> VTKPYSSPPTNLRSLRDRLTQVAERQGVVFGRLQRHV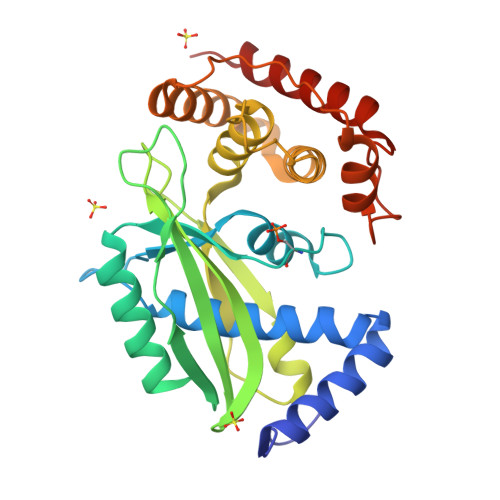AMIVVAQFAATLTDDTGAPLLLVKGGSSLELRRGIPDSRTSKDFDTVARRDIELIHEQLADAGETGWEGFTAIFTAPEEIDVPGMPVKPRRFTAKLSYRGRAFATVPIEVSSVEAGNADQFDTLTSDALGLVGVPAAVAVPCMTIPWQIAQKLHAVTAVLEEPKVNDRAHDLVDLQLLEGLLLDADLMPTRSACIAIFEARAQHPWPPRVATLPHWPLIYAGALEGLDHLELARTVDAAAQAVQRFVARIDRATKR>[12x]WNVKHDTRTLWTTPDTSPNCTIAQDKDSKLTLVLTKCGSQILANVSLIVVAGKYHIINNKNNPEIKSFTIKLLFDKNGVLLDNSN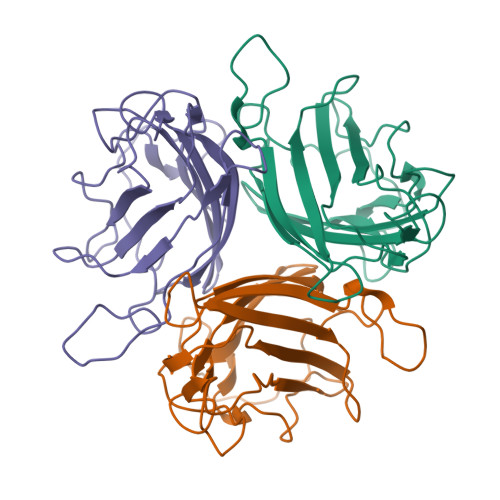LGKTYWNFRSGDSNVSTAYEKAIGFMPNLVAYPKPSNSKKYARDIVYGTIYLGGKPDQPAVIKTTFNQETGCEYSITFDFSWSKTYENVEFETTSFTFSYIAQQ[2-AMINO-3-(4-HYDROXY-PHENYL)-PROPIONYLAMINO]-(1,3,4,5-TETRAHYDROXY-4-HYDROXYMETHYL-PIPERIDIN-2-YL)- ACETIC ACID BUTYL ESTER | C21 H33 N3 O9 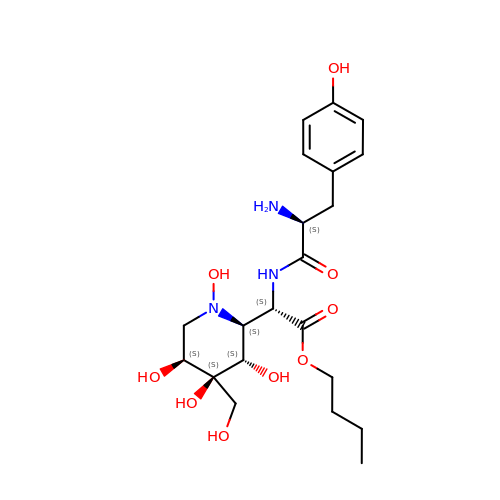| IPZUTNGJHRAITA-FULAYSDLSA-N>MADVMLNTDQINKVPNDIVTRLVRESLAEDIATGDITAQLAEDIDTTAFCITREEMILCGQDFANEVINQLDKNIQITWLYSDAQKVPANARIFELKGNVRSILTAERTILNFIQMLSGTATVTNKLVKLISQYKTKLLDTRKTIPGFRLAQKYAVRCGGGFNHRIGLFDAYLIKENHIRSAGGIAKAVTKAKKLDSNKVVEVEVTNLDELNQAIAAKADIVMLDNFSGEDIDIAVSIARGKVALEVSGNIDRNSIVAIAKTGVDFISVGAITKHIKAIDLSLQVQL[2x]

Francisella tularensis, the causative agent of tularemia, is classified by the Centers for Disease Control and Prevention (CDC) as a category A select agent, and its role as a biological weapon is known to have been investigated in the United States, the former Soviet Union, and Japan. Here, we demonstrate how a combined computational and experimental approach based on metabolic network modeling, ligand- and structure-based drug design, physiological modeling, and whole bacterial cell-based assays successfully identified novel antimicrobial compounds in a highly abbreviated time period. Third, we carried out homology modeling and X-ray crystallography to determine the structures of the selected drug targets for subsequent ligand docking. methods, three proteins [3-deoxy-d-arabino-heptulosonate-7-phosphate synthase (aroG), nicotinate-nucleotide pyrophosphorylase (nadC), and d-sedoheptulose 7-phosphate isomerase (lpcA)] were readily crystallized, and their structure was determined using molecular replacement.

We constructed and expressed full-length or slightly shortened recombinant proteins for the remaining targets to optimize protein crystallization without removing any functionally important regions. All structures were prepared as full atomistic models for use in target evaluation and ligand docking. Given computational and experimental limitations on the number of targets and compounds we could screen, we selected a diverse set of 10 candidate targets across a range of metabolic pathways. Our selected targets, as shown in Table 2, included the three enzymes we were able to crystallize (aroG, nadC, and lpcA), four protein homology model structures [shikimate kinase (aroK), pantetheine-phosphate adenylyltransferase (coaD), chorismate synthase (aroC), and 6,7-dimethyl-8-ribityllumazine synthase (ribH)], and three existing PDB crystal structures [enoyl-(acyl carrier protein) reductase (fabI), NAD synthetase (nadE), and 2-amino-4-hydroxy-6-hydroxymethyldihydropteridine pyrophosphokinase (folK)]. The success of generating crystal structures against some of these targets was greatly helped by the availability of genomic DNA, express primer service, and robotics to clone, express, and purify the proteins and to screen crystallization conditions. We mitigated these risks by considering multiple (ten) targets. This proved important because only inhibitors for roughly half the metabolic targets (four) affected bacterial growth in vivo.>[12x]AGCSDVSTELKTPVYKTKLTAEEIRNSAFKPEFPKQYASYERNDETTVMTEYKGSVPFNKNDNVNPLPEGYRHAQPYLKNLWLGYPFMYEYREARGHTYAIQDFLHIDRINRYAEKGGLPATCWNCKTPKMMEWVKESGDGFWAKDVNEFRDKIDMKDHTIGCATCHDPQTMELRITSVPLTDYLVSQGKDPKKLPRNEMRALVCGQCHVEYYFNGPTMGVNKKPVFPWAEGFDPADMYRYYDKHGDLQVKGFEGKFADWTHPASKTPMIKAQHPEYETWINGTHGAAGVTCADCHMSYTRSDDKKKISSHWW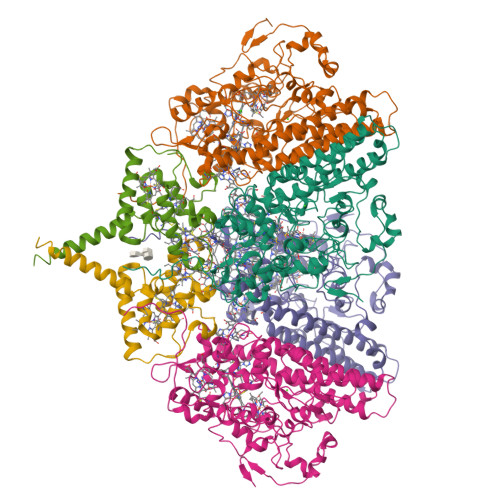TSPMKDPEMRACRQCHSDKTPDYLKSRVLFTQKRTFDLLLAAQEVSVKAHEAVRLANEYQGAKAAGYDDLMIQAREMVRKGQFFWDYVSAENSVGFHNPAKALDTLAQSQQFSQKAIDLAMEATQYGIGKDLSGDIKTIVPPILKMNRKLQQDPEFMKTHKWFQYLPVLPKADQVWDGQKRLVSAKQ;>MSEEKSRNGPARLKLVLGGATLGVVALATVAFGMKYTDQRPFCTSCHIMNPVGVTHKLSGHANISCNDCHAPHNLLAKLPFKAIAGARDVYMNTLGHPGDLILAGMETKEVVNANCKACHTMTNVEVASMEAKKYCTDCHRNVQHMRMKPISTREVADE[6x]> ASMQCKVILLDGSEYTC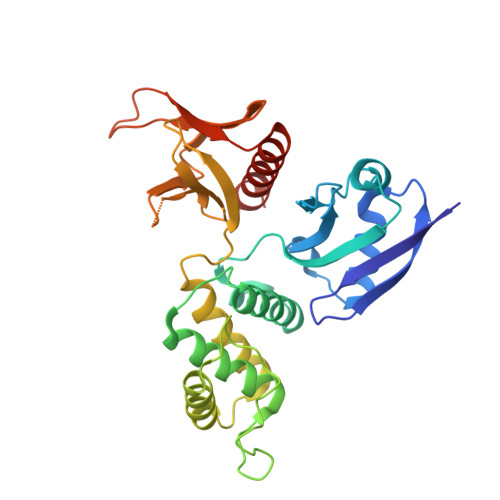DVEKRSRGQVLFDKVCEHLNLLEKDYFGLTYRDAENQKNWLDPAKEIKKQVRSGAWHFSFNVKFYPPDPAQLSEDITRYYLCLQLRDDIVSGRLPCSFVTLALLGSYTVQSELGDYDPDECGSDYISEFRFAPNHTKELEDKVIELHKSHRGMTPAEAEMHFLENAKKLSMYGVDLHHAKDSEGVEIMLGVCASGLLIYRDRLRINRFAWPKVLKISYKRNNFYIKIRPGEFEQFESTIGFKLPNHRAAKRLWKVCVEHHTFFRLL;> ARHKGTYFTHEA SUV39H1 is the first identified histone lysine methyltransferase (HMT) in human. It catalyzes di- and tri-methylation of lysine 9 of histone H3, which are related to chromatin packaging and gene silencing. SUV39H1 possesses a chromodomain at its N-terminus and a SET domain at its C-terminus. Although the SET domain performs the catalytic activity, the chromodomain of SUV39H1 is vital for the catalytic activity of SUV39H1.

However, it exists as a monomer in solution. The fold is composed of an N-terminal SH3-like β-barrel, followed by a long C-terminal helix α1(residues 82–100). The β-barrel consists of a sheet with three antiparalled strands β1 (residues 45–53), β2 (residues 58–64) and β3 (residues 73–76). Interestingly, the chromodomain of the human SUV39H1 we crystallized lacks the first aromatic residue F43 of the aromatic cage. Thus the two aromatic residues, W64 and Y67, in the loop between β2 and β3 form a partial aromatic cage, which is a conserved structural feature among chromodomain proteins and other Royal family members. This may implicate that the cage structural element is not essential for fold stability. We purified two SUV39H1 constructs including the one used for crystallization (aa 44–106) and the one containing a complete aromatic cage (aa 42–100). By means of fluorescence polarization assay, we found that the partial chromodomain does not show detectable binding to any histone H3K9 peptides.

>GEVEYLCDYKKIREQEYYLVKWRGYPDSESTWEPRQNLKCVRILKQFHKDLERELLRRHHRSKT[3x]>MSHHHHHHSMAMTQVTILKKGERITWVEVPKGESREFNIRG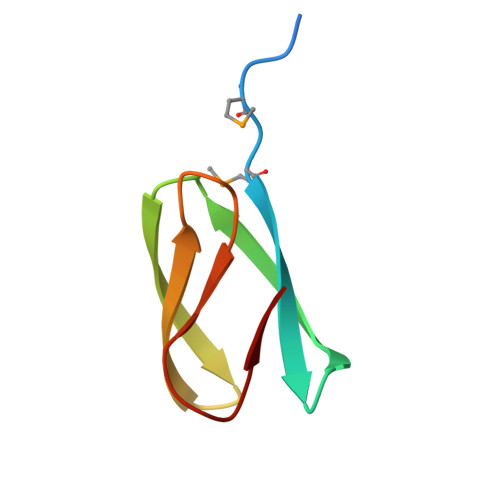KYFTVSVSDDGTPSISGSKYTVE[4x]The process is mediated by evolutionarily related signal recognition particles (SRPs) and their cognate membrane-associated receptors (SRs also called FtsYs in Bacteria and Archaea). The core proteins of SRPs and SRs are GTPases that each contain a structurally and functionally conserved NG domain where the G domain adopts a ras-like fold responsible for GTP binding and the N-domain adopts a four α-helix bundle fold. Here we describe the X-ray structures and solution conformations of FtsY, the SR from the hyper-thermophilic archaeon Pyrococcus furiosus (Pfu), in its free and GDP•magnesium-bound forms. The low resolution, solution scattering data complements our high-resolution crystallographic analysis and shows that the crystallographic structure and the average conformation adopted in solution are similar. While the overall architecture of the archeal receptor resembles its previously described bacterial homologues from the SRP/SR GTPases family, the structure of Pfu-FtsY reveals novel features: The elongated N domain lacks the N-terminal extension observed in all other bacterial FtsYs and is instead characterized by a long N-terminal helix αN1 that packs against the NG core in a different way; sequence analysis suggests that archeal receptors may cluster apart from their bacterial homologues.

The apo receptor was crystallized in two different crystallization conditions in absence of guanine nucleotide and its structure solved de novo using single wavelength anomalous dispersion of selenium; the structure is therefore not biased towards any of the previously solved homologues. Our Pfu-FtsY structure is the first representative from the Archaea kingdom. The Pfu-FtsY construct used in this study encodes the full-length receptor. The αN1 helix of Pfu-FtsY is not bent and its axis is shifted towards the core of the four α-helix bundle resulting in an overall more compact, albeit extended, N domain. In Pfu-FtsY, the N-terminus of helix αN1 is positively charged and could constitute the primary membrane interaction site supporting initial attachment of the targeting complex to the membrane and/or interaction with the membrane-embedded translocon.

> GSHMASMFGKLREKLKSFVKRVEEEVEKEEEEVEKKGLLDRILTVEIKEKDVDKALDELEIDLLEADVALEVVDALREKIKQKLVGKKVRIGTDKGKIIEEAVKEAVSEILETSRRIDLIEEIRKAEKPYVIMFVGFNGSGKTTTIAKLANWLKNHGFSVVIAASDTFRAGAIEQLEEHAKRIGVKVIKHSYGADPAAVAYDAIQHAKARGIDVVLIDTAGRSETNRNLMDEMKKIARVTKPNLVIFVGDALAGNAIVEQARQFNEAVKIDGIILTKLDADARGGAALSISYVIDAPILFVGVGQGYDDLRPFEKEWFLERIFGEENA In higher eukaryotes, a single DOT1 histone H3 lysine 79 (H3K79) methyltransferase processively produces H3K79me2/me3 through histone H2B mono-ubiquitin interaction, while the kinetoplastid Trypanosoma brucei di-methyltransferase DOT1A and tri-methyltransferase DOT1B efficiently methylate the homologous H3K76 without H2B mono-ubiquitination. DOT1 enzymes are highly conserved across metazoans and fungi, but not in the early-branched eukaryotic class of kinetoplastids including Trypanosoma brucei subsp., Trypanosoma cruzi, and Leishmania spp. In kinetoplastids, three DOT1-like methyltransferases have been identified, two of which (T. brucei DOT1A and DOT1B) have demonstrated methyltransferase activity toward H3K76 (corresponding to H3K79 in human and yeast) in vivo and in vitro. Both DOT1A and DOT1B represent minimal enzymes with less than 300 residues, comprised of a significantly diverged N-terminal domain (magenta in Fig. 1a, b) and a conserved C-terminal methyltransferase core domain (dark blue) that contains canonical and non-canonical methyltransferase motifs. Based on structural and biochemical analyses of DOT1A, we identify key residues in the methyltransferase motifs VI and X for efficient ubiquitin-independent H3K76 methylation in kinetoplastids. Substitution of a basic to an acidic residue within motif VI (Gx6K) is essential to stabilize the DOT1A enzyme-substrate complex, while substitution of the motif X sequence VYGE by CAKS renders a rigid active-site loop flexible, implying a distinct mechanism of substrate recognition.

To investigate the implications of these differences on the structural level, we determined the X-ray crystal structure of DOT1A and compared it to human and yeast active-form DOT1-nucleosome complexes. Δ42-DOT1A crystallized in complex with the methyl donor product AdoHcy in two different crystal forms (space groups C2221 and P212121), and their structures were determined at 2.1 and 1.9 Å resolution, respectively. The asymmetric units of the C2221 and P212121 space groups contain one and two DOT1A enzymes referred to as Molecules I to III, respectively. All three molecules are highly similar with a root-mean-square deviation (rmsd) of ~0.3 Å comparing 234 pairs of Cα atoms. The methyltransferase motifs I, II, and III are highly conserved among DOT1 enzymes including DOT1A and DOT1B, and electron density of AdoHcy in the crystal structures of DOT1A are clearly observed in all three molecules. Specifically, AdoHcy is recognized by DOT1A Asp134 (motif I), the Gly136 main chain (motif I), Glu158 (motif II), Met196 (motif III), and Phe222 (adjacent to motif IV). In DOT1A molecules I and II of the two crystal forms, the CAKS sequence-containing loop FH lacks electron density and is disordered, implying flexibility. In DOT1A molecule III, this loop is ordered (colored in purple), which is likely due to stabilization by a symmetry-related molecule in the crystal.

>[2x]GPHMPKGELGAGTPHEPYNLPLRGNPNKSGCHHCLADQCHCVFFERLLDATFRRLDIKRITEVSGSRHLCAKSLLPTFVSRMVRLMEITSEDTFYDLGCGNGSILFQVAFLTGARCVGIEISEHNAKVAKKAWEVIRPELEGSSGRSMSEVNIITSDMTKILADERLFESERGKTVILLSNLLFPKSLTHYLSERFRRVPSGTRILCFDDLYPHSRSVAAIRDPEAFRLFAMTDYRWQECSVEWCTRDGPFFIHRRR> SNAEDITETSPDKWLIDGDTPLDEVERAIGYELPEGDYETISGLLFDHANALLKTGDVIEIPLDF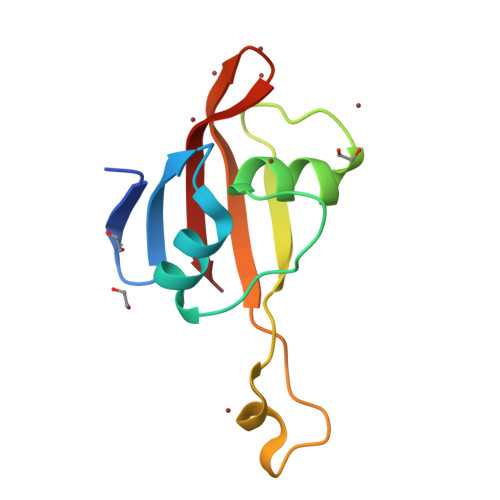EPEDYLNNTSPTQRILRITVLEVERNVPVKLALALL> MVTREEFVARFGGVFEHSPFIAERAYDAGGAGLELTAKAVHGALCAQFRVASEAERLGVLRAHPDLAGKLAIAGELTADSRNEQAGAGLDRLSPQEHARFTQLNSAYTEKFGFPFIIAVKGLNR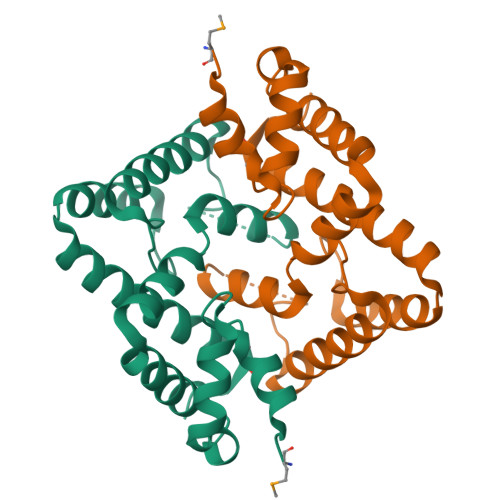HDILSAFDTRIDNNAAQEFATATGQVEKIAWLRLASMLPEG>[4x]QRKLEAL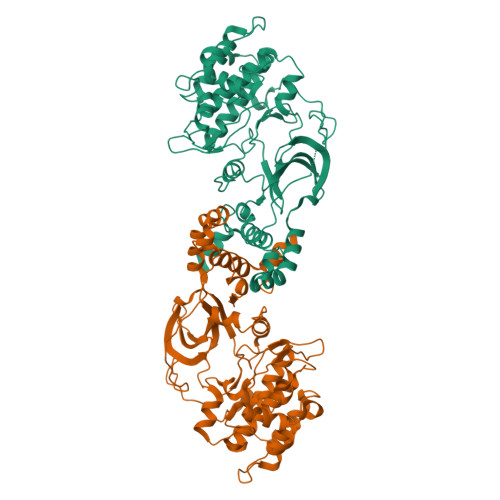IRDPRSPINVESLLDGLNSLVLDLDFPALRKNKNIDNFLNRYEKIVKKIRGLQMKAEDYDVVKVIGRGAFGEVQLVRHKASQKVYAMKLLSKFEMIKRSDSAFFWEERDIMAFANSPWVVQLFCAFQDDKYLYMVMEYMPGGDLVNLMSNYDVPEKWAKFYTAEVVLALDAIHSMGLIHRDVKPDNMLLDKHGHLKLADFGTCMKMDETGMVHCDTAVGTPDYISPEVLKSQGGDGYYGRECDWWSVGVFLFEMLVGDTPFYADSLVGTYSKIMDHKNSLCFPEDAEISKHAKNLICAFLTDREVRLGRNGVEEIKQHPFFKNDQWNWDNIRETAAPVVPELSSDIDSSNFDDIEDDKGDVETFPIPKAFVGNQLPFIGFTYYR> GSHMEDYNFVFKVVLIGESGVGKTNLLSRFTRNEFSHDSRTTIGVEFSTRTVMLGTAAVKAQIWDTAGLERYRAITSAYYRGAVGALLV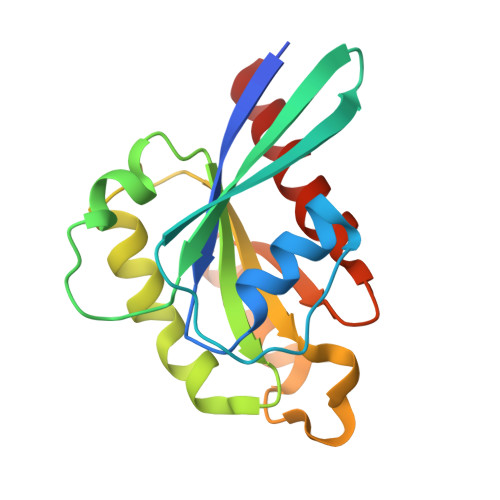FDLTKHQTYAVVERWLKELYDHAEATIVVMLVGNKSDLSQAREVPTEEARMFAENNGLLFLETSALDSTNVELAFETVLKEIFAKVSKQ> MDPYCPFDALDVWEHRRFIVADSRNFITPEFPRDFWMSPVFNLPRETAAEQVVVLQAQRTAAAAALENAAMQAAELPV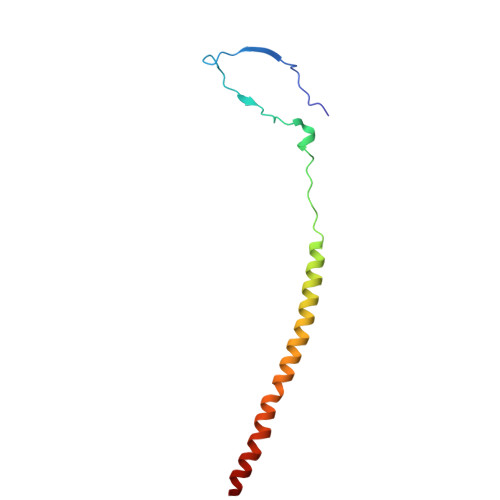DIERRLRPIERNVHEI>NNEIIPGKLKQRSIKAEGDGIVGEGKALYNNEGGRTFMYAFISDKPDLRVVKWEFDGGANTIELEPPRKFLVDSPNGAQIKYLYFVRNLNTLR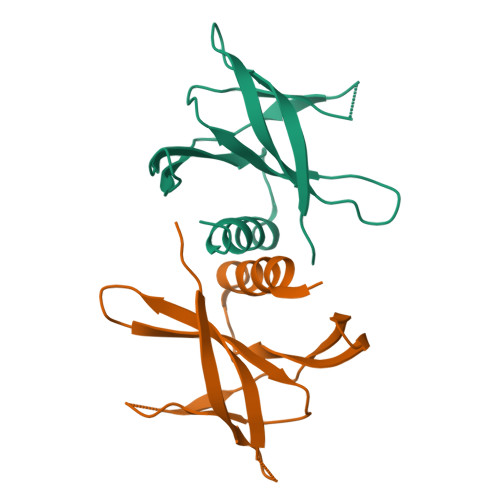RGAVLGYIGATVRLQHHHHHH[3x]The S. cerevisiae Neo1 and its orthologs represent the P4B ATPases, which function as monomeric flippases without a β-subunit. Here we report the structure of a P4B ATPase, Neo1, in its E1-ATP, E2P-transition, and E2P states. The structure reveals a conserved architecture as well as highly similar functional intermediate states relative to dimeric flippases. Most P-type ATPases have a conserved architecture consisting of a transmembrane domain (TMD), an actuator domain (A-domain), a nucleotide-binding domain (N-domain), and a phosphorylation domain (P-domain).

We obtained cryo-EM 3D maps of Neo1 in the E1-ATP state stabilized by AMPPCP at 5.6-Å resolution, in the E2P-transition state of dephosphorylation stabilized by AlF4− at the 3.1-Å resolution, and in the E2P state as stabilized by BeF3− at 3.2-Å resolution. The bound AlF4− and BeF3− mimic the planar pentavalent transition state of phosphoryl transfer and the covalent phosphorylated E2P ground state, respectively. We first built atomic models into the 3.2-Å resolution map in the E2P state and into the 3.1-Å resolution map in the E2P-transition state. The phosphorylated aspartate is mimicked by the BeF3− moiety in our Neo1 structure. To enter into the E2P state, both the N and A domains swing away from the membrane and pack tightly together. Accompanying this transition, the TMH2 becomes straightened, pointing downwards to allow the A domain movement. Comparison of the Neo1 structures in the E1-ATP and the E2P states shows that the whole TMD and the P domain are superimposable, while the N and A domains have undergone dramatic conformational changes. Furthermore, the conformation and the substrate transport path of Neo1 in the E2P state highly resemble those of the Drs2, Dnf1, ATP8A1, and ATP11C flippases in the same E2P state. A structure-based homology search revealed that Neo1 in the E2P state aligned well with all known P4 ATPase structures in that state, but the best match was with Dnf1. Previous reported Dnf1 structure contained phospholipid molecules in both the substrate entry and exit sites, but we did not capture any endogenous lipid molecules in the Neo1 substrate sites.

> MPNPPSFKSHKQNLFNSNNNQHANSVDSFDLHLDDSFDAALDSLQINNNPEPLSKHNTVGDRESFEMRTVDDLDNFSNHSSDSHRKSSNTDTHPLMYDNRLSQDDNFKFTNIASSPPSSSNNIFSKALSYLKVSNTKNWSKFGSPIELSDQHIEREIHPDTTPVYDRNRYVSNELSNAKYNAVTFVPTLLYEQFKFFYNLYFLVVALSQAVPALRIGYLSSYIVPLAFVLTVTMAKEAIDDIQRRRRDRESNNELYHVITRNRSIPSKDLKVGDLIKVHKGDRIPADLVLLQSSEPSGESFIKTDQLDGETDWKLRVACPLTQNLSENDLINRISITASAPEKSIHKFLGKVTYKDSTSNPLSVDNTLWANTVLASSGFCIACVVYTGRDTRQAMNTTTAKVKTGLLELEINSISKILCACVFALSILLVAFAGFHNDDWYIDILRYLILFSTIIPVSLRVNLDLAKSVYAHQIEHDKTIPETIVRTSTIPEDLGRIEYLLSDKTGTLTQNDMQLKKIHLGTVSYTSETLDIVSDYVQSLVSSKNDSLNNSKVALSTTRKDMSFRVRDMILTLAICHNVTPTFEDDELTYQAASPDEIAIVKFTESVGLSLFKRDRHSISLLHEHSGKTLNYEILQVFPFNSDSKRMGIIVRDEQLDEYWFMQKGADTVMSKIVESNDWLEEETGNMAREGLRTLVIGRKKLNKKIYEQFQKEYNDASLSMLNRDQQMSQVITKYLEHDLELLGLTGVEDKLQKDVKSSIELLRNAGIKIWMLTGDKVETARCVSISAKLISRGQYVHTITKVTRPEGAFNQLEYLKINRNACLLIDGESLGMFLKHYEQEFFDVVVHLPTVIACRCTPQQKADVALVIRKMTGKRVCCIGDGGNDVSMIQCADVGVGIVGKEGKQASLAADFSITQFCHLTELLLWHGRNSYKRSAKLAQFVMHRGLIIAICQAVYSICSLFEPIALYQGWLMVGYATCYTMAPVFSLTLDHDIEESLTKIYPELYKELTEGKSLSYKTFFVWVLLSLFQGSVIQLFSQAFTSLLDTDFTRMVAISFTALVVNELIMVALEIYTWNKTMLVTEIATLLFYIVSVPFLGDYFDLGYMTTVNYYAGLLVILLISIFPVWTAKAIYRRLHPPSYAKVQEFATP>MAFQLEMVTRETVVIRLFGELDHHAVEQIRAKISTAIFQGAVTTIIWNFERLSFMDSSGVGLVLGRMRELEAVAGRTILLNPS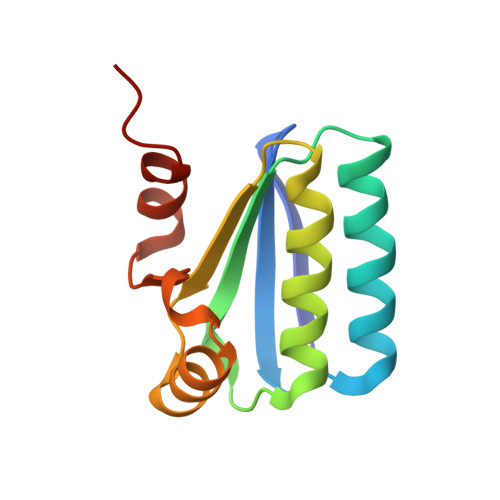PTVRKVFQFSGLGPWMMDATEEEAIDRVRGIVNG[2x]> MRLFVSDGVPGCLPVLAAAGRARGRAEVLISTVGPQDCVVPFLTRPKVPVLQLDSGNYLFSTSAICRYFFLLSGWEQDDLTNQWLEWEATELQPALSAALYYLVVQGKKGEDVLGSVRRALTHIDHSLSRQNCPFLAGETESLADIVLWGALYPLLQDPAYLPEELSALHSWFQTLSTQ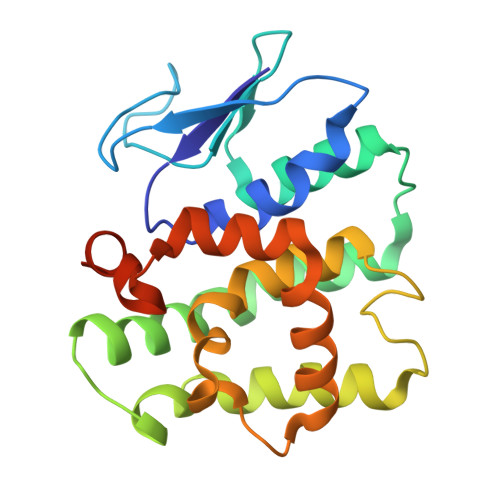EPCQRAAQTVLKQQGVLALRPYLQKQPQLEHHHHHH>[2x]MRGSHHHHHHGMASMRILLSNDDGVHAPGIQTLAKALREFADVQVVAPDRNRSGASNSLT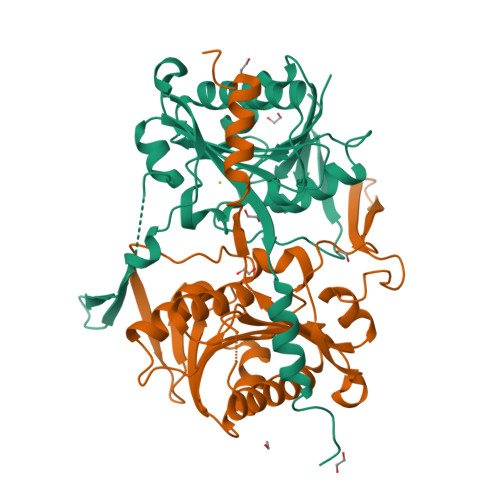LESSLRTFTFDNGDIAVQMGTPTDCVYLGVNALMRPRPDIVVSGINAGPNLGDDVIYSGTVAAAMEGRHLGFPALAVSLNGYQHYDTAAAVTCALLRGLSREPLRTGRILNVNVPDLPLAQVKGIRVTRCGSRHPADKVIPQEDPRGNTLYWIGPPGDKYDAGPDTDFAAVDEGYVSVTPLHVDLTAASAHDVVSDWLDSVGVGTQW>[3x]MEGVVRLEVPTPEEGFVNITRKVEAALSGHTGLVYLFVPHTTCGLTVQEGADPTVAQDLLGRLAELAPRHRPQDRHLEGNSHAHLKSLLTG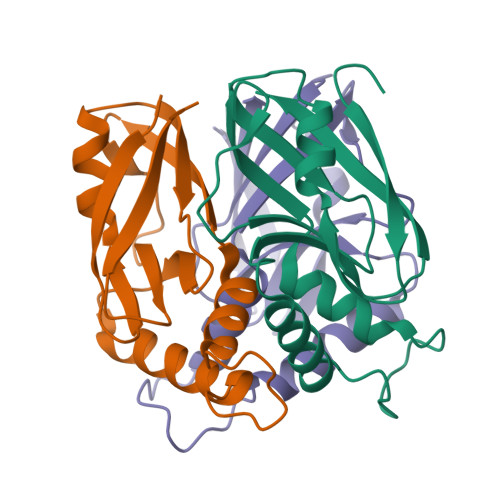VHLLLLAEKGRLRLGRWQQVFLAEFDGPRVREVWVRLL> GAMGNQTVKIWVKYNEGFSNAVR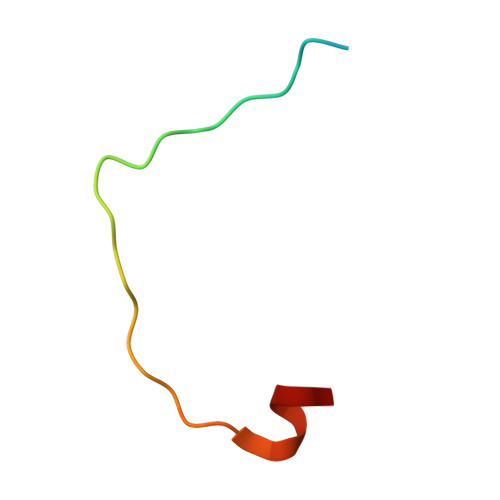KNVTWNNLWE(2S)-3-acetyloxy-2-[(E)-[2-methyl-3-oxidanyl-5-(phosphonooxymethyl)pyridin-4-yl]methylideneamino]propanoic acid | C13 H17 N2 O9 P 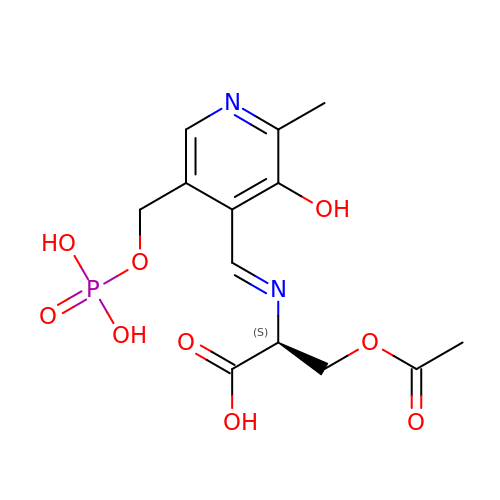| CDKXKQFHRCVQDP-WCFOZWBASA-N>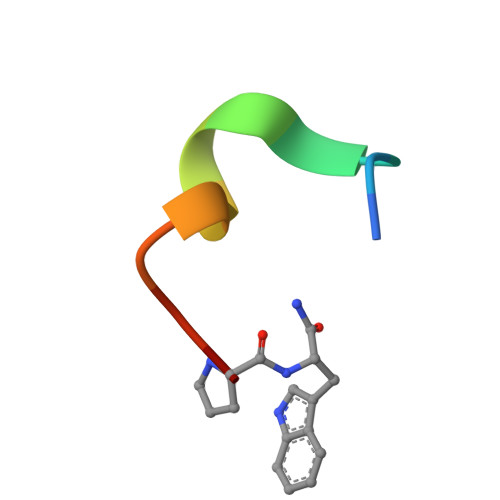 TCVNIMCCRCPX> DDVSISPEQSFYEIMLIRPKTIDDINYVVDQVLEESNPVILDLSFLE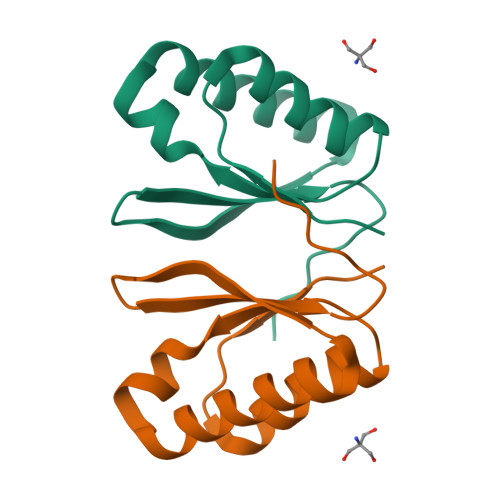KESPANFKLAGEKIKQMRSNYGAEALLLSRCNDKNLIIIAPKGVSLVRK> MKRVVITGLGIVSSIGNNQQEVLASLREGRSGITFSQELKDSGMRSHVWGNVKLDTTGLIDRKVVRFMSDASIYAFLSMEQAIADAGLSPEAYQNNPRVGLIAGSGGGSPRFQVFGADAMRGPRGLKAVGPYVVTKAMASGVSACLATPFKIHGVNYSISSACATSAHCIGNAVEQIQLGKQDIVFAGGGEELCWEMACEFDAMGALSTKYNDTPEKASRTYDAHRDGFVIAGGGGMVVVEELEHALARGAHIYAEIVGYGATSDGADMVAPSGEGAVRCMKMAMHGVDTPIDYLNSHGTSTPVGDVKELAAIREVFGDKSPAISATKAMTGHSLGAAGVQEAIYSLLMLEHGFIAPSINIEELDEQAAGLNIVTETTDRELTTVMSNSFGFGGTNATLVMRKLK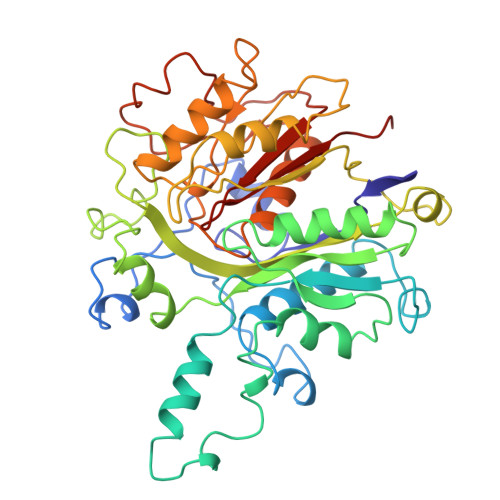D PYRIMIDINE-2,4-DIAMINE | C4 H6 N4 | 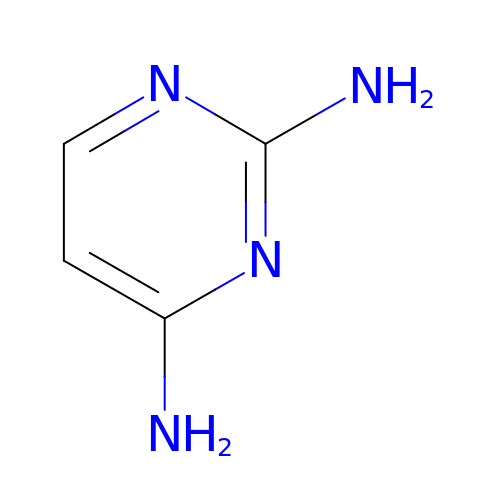YAAWASYJIRZXSZ-UHFFFAOYSA-N> SKTITIYLDHASLPTLNQLMHFTKESEDKETARIFGFSRFKLPEKITEQYNNIHFVEIKNNRPTEDIFTILDQYPEKLELDLHL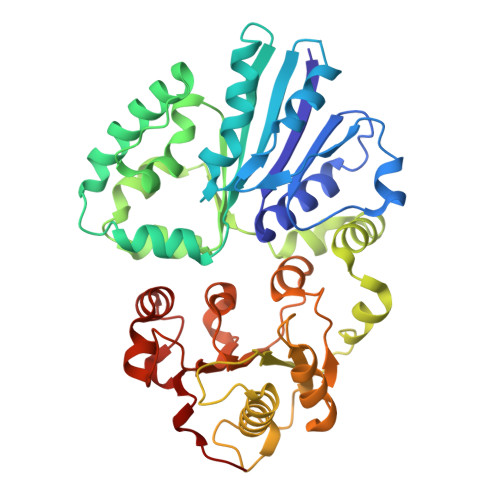NIAHSIQLFHPILQYRFKHPDRISIKSLNLYDDGTAEYVDLEKEENKDIKSAIKKAEKQLSDYLLTGKINFDNPTLARYVWQSQYPVKYHFLSTEYFEKAEFLQPLKTYLAGKYQKMDWSAYEKLSPEQQTFYLKLVGFSDETKQLFHTEQTKFIFTGTTTWEGNTDIREYYAKQQLNLLKHFTHSEGDLFIGDQYKIYFKGHPRGGDINDYILKHAKDITNIPANISFEILMMTGLLPDKVGGVASSLYFSLPKEKISHIIFTSNKKIKNKEDALNDPYVRVMLRLGMIDKSQIIFWDSLKQL For example, in the yeast S. cerevisiae, these supercomplexes are composed of a CIII2 dimer flanked by one or two copies of CIV (CIII2CIV1/2). Complex III2 is an obligate dimer, which receives electrons from membrane-bound ubiquinol (QH2). In CIV, electrons are first transferred to a di-nuclear CuA site, located on the p-side of CIV, and then consecutively to heme a and the heme a3-CuB catalytic site where molecular oxygen binds and is reduced to water. Electron transfer between CIII2 and CIV is mediated via soluble cyt. c.

We mixed the supercomplex and cyt. c at a ~ 1:12 ratio ( ~ 10 µM supercomplex) in a solution with an ionic strength of 20 mM and applied the sample to holey gold grids for analysis by cryo-EM. Analysis of the resulting three-dimensional (3D) maps showed a CIII2 dimer flanked by either one or two monomers of CIV, consistent with earlier observations. Combining the CIII2CIV2 and CIII2CIV1 particle images for refinement led to a map with a nominal resolution of 2.4 Å. Densities originating from nine water molecules are seen in the D proton pathway in subunit Cox1 of CIV, which connects the highly conserved Asp92 on the n side with another conserved protonatable residue, Glu243, from where protons are transferred either to the catalytic site after binding of O2 or are pumped toward the p-side of the membrane. In addition, two water molecules were identified in the K proton pathway, which connects Glu82, near the n-side surface of subunit Cox2, via the conserved Lys319 (Cox1), with the catalytic site. However, in contrast to the earlier S. cerevisiae supercomplex models, we identified a cardiolipin (CL) at a site previously modeled as two phosphatidylethanolamine (PE) lipid molecules, which is similar to the CL identified in Yarrowia lipolytica CIII247. As in our previous study performed at 150 mM KCl30, we detected an elongated density corresponding to cyt. c bound at different locations on the negatively charged p-side surface of the supercomplex, spanning between cyt. c1 on each CIII in CIII2 and CuA on CIV. We also observed density that is attributed to 7-8-amino-acid residues C-terminal segment of subunit Qcr9, which interacts with cyt. c bound at CIV. The C-terminal sequence from Qcr9 is also composed of a majority (~ 80%) negatively charged residues, which would explain why it could not be observed in the absence of cyt. c.

>[2x]AEVTQLSNGIVVATEHNPSAHTASVGVVFGSGAANENPYNNGVSNLWKNIFLSKENSAVAAKEGLALSSNISRDFQSYIVSSLPGSTDKSLDFLNQSFIQQKANLLSSSNFEATKKSVLKQVQDFEENDHPNRVLEHLHSTAFQNTPLSLPTRGTLESLENLVVADLESFANNHFLNSNAVVVGTGNIKHEDLVNSIESKNLSLQTGTKPVLKKKAAFLGSEVRLRDDTLPKAWISLAVEGEPVNSPNYFVAKLAAQIFGSYNAFEPASRLQGIKLLDNIQEYQLCDNFNHFSLSYKDSGLWGFSTATRNVTMIDDLIHFTLKQWNRLTISVTDTEVERAKSLLKLQLGQLYESGNPVNDANLLGAEVLIKGSKLSLGEAFKKIDAITVKDVKAWAGKRLWDQDIAIAGTGQIEGLLDYMRIRSDMSMMRW;>[2x]LTVSARDAPTKISTLAVKVHGGSRYATKDGVAHLLNRFNFQNTNTRSALKLVRESELLGGTFKSTLDREYITLKATFLKDDLPYYVNALADVLYKTAFKPHELTESVLPAARYDYAVAEQCPVKSAEDQLYAITFRKGLGNPLLYDGVERVSLQDIKDFADKVYTKENLEVSGENVVEADLKRFVDESLLSTLPAGKSLVSKSEPKFFLGEENRVRFIGDSVAAIGIPVNKASLAQYEVLANYLTSALSELSGLISSAKLDKFTDGGLFTLFVRDQDSAVVSSNIKKIVADLKKGKDLSPAINYTKLKNAVQNESVSSPIELNFDAVKDFKLGKFNYVAVGDVSNLPYLDEL;>MAFRKSNVYLSLVNSYIIDSPQPSSINYWWNMGSLLGLCLVIQIVTGIFMAMHYSSNIELAFSSVEHIMRDVHNGYILRYLHANGASFFFMVMFMHMAKGLYYGSYRSPRVTLWNVGVIIFILTIATAFLGYCCVYGQMSHWGATVITNLFSAIPFVGNDIVSWLWGGFSVSNPTIQRFFALHYLVPFIIAAMVIMHLMALHIHGSSNPLGITGNLDRIPMHSYFIFKDLVTVFLFMLILALFVFYSPNTLGHPDNYIPGNPLVTPASIVPEWYLLPFYAILRSIPDKLLGVITMFAAILVLLVLPFTDRSVVRGNTFKVLSKFFFFIFVFNFVLLGQIGACHVEVPYVLMGQIATFIYFAYFLIIVPVISTIENVLFYIGRVNK[2x];>MTAAEHGLHAPAYAWSHNGPFETFDHASIRRGYQVYREVCAACHSLDRVAWRTLVGVSHTNEEVRNMAEEFEYDDEPDEQGNPKKRPGKLSDYIPGPYPNEQAARAANQGALPPDLSLIVKARHGGCDYIFSLLTGYPDEPPAGVALPPGSNYNPYFPGGSIAMARVLFDDMVEYEDGTPATTSQMAKDVTTFLNWCAEPEHDERKRLGLKTVIILSSLYLLSIWVKKFKWAGIKTRKFVFNPPKPR[2x];>KSTYRTPNFDDVLKENNDADKGRSYAYFMVGAMGLLSSAGAKSTVETFISSMTATADVLAMAKVEVNLAAIPLGKNVVVKWQGKPVFIRHRTPHEIQEANSVDMSALKDPQTDADRVKDPQWLIMLGICTHLGCVPIGEAGDFGGWFCPCHGSHYDISGRIRKGPAPLNLEIPAYEFDGDKVIVG[2x];>EVTDQLEDLREHFKNTEEGKALVHHYEECAERVKIQQQQPGYADLEHKEDCVEEFFHLQHYLDTATAPRLFDKLK[2x];>[2x]PQSFTSIARIGDYILKSPVLSKLCVPVANQFINLAGYKKLGLKFDDLIAEENPIMQTALRRLPEDESYARAYRIIRAHQTELTHHLLPRNEWIKAQEDVPYLLPYILEAEAAAKEKDELDNIEVSK;>GPPSGKTYMGWWGHMGGPKQKGITSYAVSPYAQKPLQGIFHNAVFNSFRRFKSQFLYVLIPAGIYWYWWKNGNEYNEFLYSKAGREELERVNV[2x];>SFSSLYKTFFKRNAVFVGTIFAGAFVFQTVFDTAITSWYENHNKGKLWKDVKARIAA[2x];>AYTSHLSSKTGLHFGRLSLRSLTAYAPNLMLWGGASMLGLFVFTEGWPKFQDTLYKKIPLLGPTLEDHTPPEDKPN[2x];> MVQRWLYSTNAKDIAVLYFMLAIFSGMAGTAMSLIIRLELAAPGSQYLHGNSQLFNVLVVGHAVLMIFFLVMPALIGGFGNYLLPLMIGATDTAFPRINNIAFWVLPMGLVCLVTSTLVESGAGTGWTVYPPLSSIQAHSGPSVDLAIFALHLTSISSLLGAINFIVTTLNMRTNGMTMHKLPLFVWSIFITAFLLLLSLPVLSAGITMLLLDRNFNTSFFEVSGGGDPILYEHLFWFFGHPEVYILIIPGFGIISHVVSTYSKKPVFGEISMVYAMASIGLLGFLVWSHHMYIVGLDADTRAYFTSATMIIAIPTGIKIFSWLATIHGGSIRLATPMLYAIAFLFLFTMGGLTGVALANASLDVAFHDTYYVVGHFHYVLSMGAIFSLFAGYYYWSPQILGLNYNEKLAQIQFWLIFIGANVIFFPMHFLGINGMPRRIPDYPDAFAGWNYVASIGSFIATLSLFLFIYILYDQLVNGLNNKVNNKSVIYNKAPDFVESNTIFNLNTVKSSSIEFLLTSPPAVHSFNTPAVQS;> DVPTPYACYFQDSATPNQEGILELHDNIMFYLLVILGLVSWMLYTIVMTYSKNPIAYKYIKHGQTIEVIWTIFPAVILLIIAFPSFILLYLCDEVISPAMTIKAIGYQWYWKYEYSDFINDSGETVEFESYVIPDELLEEGQLRLLDTDTSMVVPVDTHIRFVVTAADVIHDFAIPSLGIKVDATPGRLNQVSALIQREGVFYGACSELCGTGHANMPIKIEAVSLPKFLEWLNEQ;> MTHLERSRHQQHPFHMVMPSPWPIVVSFALLSLALSTALTMHGYIGNMNMVYLALFVLLTSSILWFRDIVAEATYLGDHTMAVRKGINLGFLMFVLSEVLIFAGLFWAYFHSAMSPDVTLGACWPPVGIEAVQPTELPLLNTIILLSSGATVTYSHHALIAGNRNKALSGLLITFWLIVIFVTCQYIEYTNAAFTISDGVYGSVFYAGTGLHFLHMVMLAAMLGVNYWRMRNYHLTAGHHVGYETTIIYTHVLDVIWLFLYVVFYWWGV;> VVKTAQNLAEVNGPETLIGPGAKEGTVPTDLDQETGLARLELLGKLEGIDVFDTKPLDSSRKGTMKDPIIIESYDDYRYVGCTGSPAGSHTIMWLKPTVNEVARCWECGSVYKLNPVGVP;> AQTHALSNAAVMDLQSRWENMPSTEQQDIVSKLSERQKLPWAQLTEPEKQAVWYISYGEWGPRRPVLNKGDSSFIAKGVAAGLLFSVGLFAVVRMAGGQDAKTMNKEWQLKSDEYLKSKNANPWGGYSQVQSK;> DEETFEEFTARYEKEFDEAYDLFEVQRVLNNCFSYDLVPAPAVIEKALRAARRVNDLPTAIRVFEALKYKVENEDQYKAYLDELKDVRQELGVPLKEELFPS;> ANKVIQLQKIFQSSTKPLWWRHPRSALYLYPFYAIFAVAVVTPLLYIPNAIRGIKAKKA;> VHFKDGVYENIPFKVKGRKTPYALSHFGFFAIGFAVPFVACYVQLKKSGAF;> TIAPITGTIKRRVIMDIVLGFSLGGVMASYWWWGFHMDKINKREKFYAELAERKK;> SPLHTVGFDARFPQQNQTKHCWQSYVDYHKCVNMKGEDFAPCKVFWKTYNALCPLDWIEKWDDQREKGIFAGDIN;> LPPNALKPAFGPPDKVAAQKFKESLMATEKHAKDTSNMWVKISVWVALPAIALTAVNTYFVEKEHAEHREHLKHVPDSEWPRDYEFMNIRSKPFFWGDGDKTLFWNPVVNRHI;> GRIGESWVITEGRRLIPEIFQWSAVLSVCLGWPGAVYFFSKARKA(2E)-3-{5-[(2,4-diaminopyrimidin-5-yl)methyl]-2,3-dimethoxyphenyl}-1-[(1S)-1-(3,3,3-trifluoropropyl)phthalazin-2(1H)-yl]prop-2-en-1-one 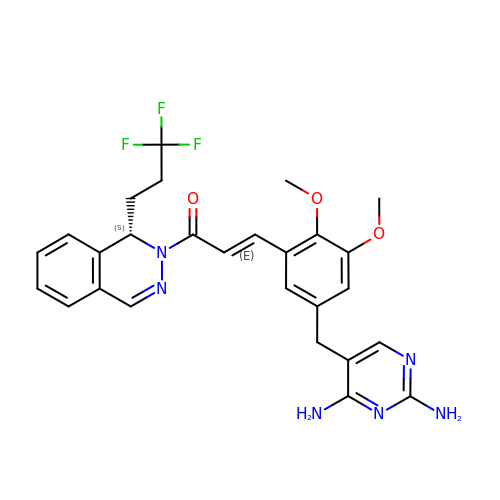| C27 H27 F3 N6 O3 | YOZBLXHLSFVRNH-CQQBXOTJSA-N>[2x]STHFDVIVVGAGSMGMAAGYQLAKQGVKTLLVDAFDPPHTNGSHHGDTRIIRHAYGEGREYVPLALRSQELWYELEKETHHKIFTKTGVLVFGPKGESAFVAETMEAAKEHSLTVDLLEGDEINKRWPGITVPENYNAIFEPNSGVLFSENCIRAYRELAEARGAKVLTHT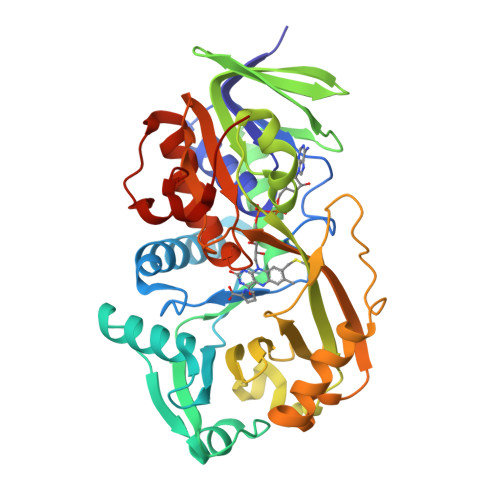RVEDFDISPDSVKIETANGSYTADKLIVSMGAWNSKLLSKLNLDIPLQPYRQVVGFFESDESKYSNDIDFPGFMVEVPNGIYYGFPSFGGCGLKLGYNTFGQKIDPDTINREFGVYPEDESNLRAFLEEYMPGANGELKRGAVCMYTKTLDEHFIIDLHPEHSNVVIAAGFSGHGFKFSSGVGEVLSQLALTGKTEHDISIFSINRPALKESLQKTTI>[2x]MRIIMPVEFSRIVRDVERLIAVEKYSLQGVVDGDKLLVVGFSEGSVNAYLYDGGETVKLNREPINSVLDPHYGVGRVILVRDVSKGAEQHALFKVNTSRPGEEQRL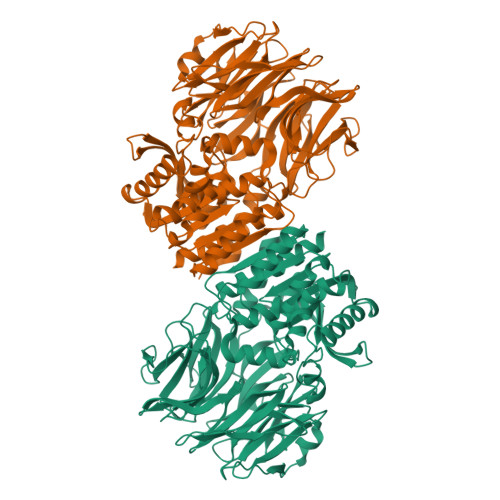EAVKPMRILSGVDTGEAVVFTGATEDRVALYALDGGGLRELARLPGFGFVSDIRGDLIAGLGFFGGGRVSLFTSNLSSGGLRVFDSGEGSFSSASISPGMKVTAGLETAREARLVTVDPRDGSVEDLELPSKDFSSYRPTAITWLGYLPDGRLAVVARREGRSAVFIDGERVEAPQGNHGRVVLWRGKLVTSHTSLSTPPRIVSLPSGEPLLEGGLPEDLRRSIAGSRLVWVESFDGSRVPTYVLESGRAPTPGPTVVLVAGGPFAEDSDSWDTFAASLAAAGFHVVMPNYRGSTGYGEEWRLKIIGDPCGGELEDVSAAARWARESGLASELYIMGYSYGGYMTLCALTMKPGLFKAGVAGASVVDWEEMYELSDAAFRNFIEQLTGGSREIMRSRSPINHVDRIKEPLALIHPQNDSRTPLKPLLRLMGELLARGKTFEAHIIPDAGHAINTMEDAVKILLPAVFFLATQRERR> LGSGCHHRICHCSNRVFLCQESKVTEIPSDLPRNAIELRFVLTKLRVIQKGAFSGFGDLEKIEISQNDVLEVIEADVFSNLPKLHEIRIEKANNLLYINPEAFQNLPNLQYLLISNTGIKHLPDVHKIHSLQKVLLDIQ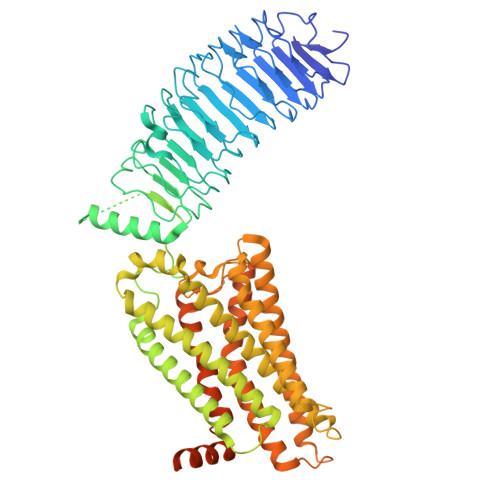DNINIHTIERNSFVGLSFESVILWLNKNGIQEIHNCAFNGTQLDELNLSDNNNLEELPNDVFHGASGPVILDISRTRIHSLPSYGLENLKKLRARSTYNLKKLPTLEKLVALMEASLTYPSHCCAFANWRRQISELHPICNKSILRQEVDYMTQARGQRSSLAEDNESSYSRGFDMTYTEFDYDLCNEVVDVTCSPKPDAFNPCEDIMGYNILRVLIWFISILAITGNIIVLVILTTSQYKLTVPRFLMCNLAFADLCIGIYLLLIASVDIHTKSQYHNYAIDWQTGAGCDAAGFFTVFASELSVYTLTAITLERWHTITHAMQLDCKVQLRHAASVMVMGWIFAFAAALFPIFGISSYMKVSICLPMDIDSPLSQLYVMSLLVLNVLAFVVICGCYIHIYLTVRNPNIVSSSSDTRIAKRMAMLIFTDFLCMAPISFFAISASLKVPLITVSKAKILLVLFHPINSCANPFLYAIFTKNFRRDFFILLSKCGCYEMQAQIYRTETSSTVHNTHPRNGHCSSAPRVTNGSTYILVPLSHLAQN>[4x]MSKPIEIEIRRAPVLGSSMAYRETGAQDAPVVLFLHGNPTSSHIWRNILPLVSPVAHCIAPDLIGFGQSGKPDIAYRFFDHVRYLDAFIEQRGVTSAYLVAQDWGTALAFHLAARRPDFVRGLAFMEFIRPMPTWQDFHHTEVAEEQDHAEAAR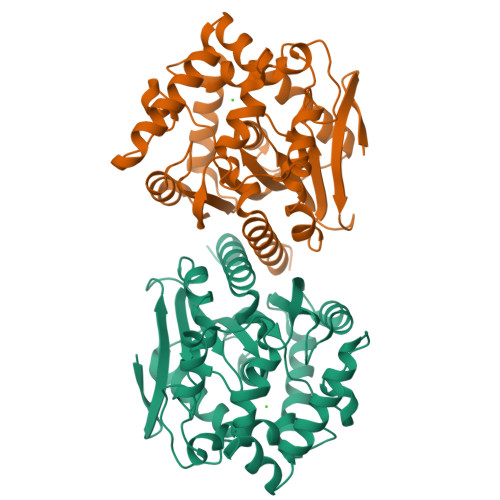AVFRKFRTPGEGEAMILEANAFVERVLPGGIVRKLGDEEMAPYRTPFPTPESRRPVLAFPRELPIAGEPADVYEALQSAHAALAASSYPKLLFTGEPGALVSPEFAERFAASLTRCALIRLGAGLHYLQEDHADAIGRSVAGWIAGIEAVRPQLAAVD> PAPHGGILQDLIARDALKKNELLSEAQSSDILVWNLTPRQLCDIELILNGGFSPLTGFLNENDYSSVVTDSRLADGTLWTIPITLDVDEAFANQIKPDTRIALFQDDEIPIAILTVQDVYKPNKTIEAEKVFRGDPEHPAISYLFNVAGDYYVGGSLEAIQLPQHYDYPGLRKTPAQLRLEFQSRQWDRVVAFQTRNPMHRAHRELTVRAAREANAKVLIHPVVGLTKPGDIDHHTRVRVYQEIIKRYPNGIAFLSLLPLAMRMSGDREAVWHAIIRKNYGASHFIVGRDHAGPGKNSKGVDFYGPYDAQELVESYKHELDIEVVPFRMVTYLPDEDRYAPIDQIDTTKTRTLNISGTELRRRLRVGGEIPEW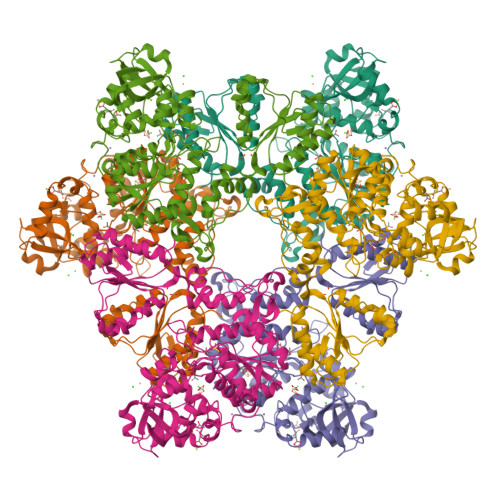FSYPEVVKILRESNPPRPKQGFSIVLGNSLTVSREQLSIALLSTFLQFGGGRYYKIFEHNNKTELLSLIQDFIGSGSGLIIPNQWEDDKDSVVGKQNVYLLDTSSSADIQLESADEPISHIVQKVVLFLEDNGFFVF The main protease (Mpro) of the betacoronavirus SARS-CoV-2 is an attractive target for the development of treatments for COVID-19. Starting from crystal structures of the Mpro in complexes with the Hepatitis C virus NS3/4A protease inhibitors boceprevir and telaprevir, we optimized the potency of the alpha-ketoamide boceprevir against the Mpro by replacing its P1 cyclobutyl moiety by a γ-lactam as a glutamine surrogate. In line with our original goal of identifying broad-spectrum inhibitors that target the main protease of coronaviruses and the 3C protease of enteroviruses, we also assessed the inhibitory potency of MG-78 against the Mpro of the alphacoronavirus HCoV NL63 and the 3Cpros of enterovirus A71 (EV-A71) and Coxsackievirus B3 (CVB3). Finally, coronavirus Mpros feature a catalytic dyad comprising a Cys…His pair, whereas enterovirus 3Cpros have a catalytic triad consisting of Cys…His…Glu(Asp).

Using 10 µM Dabcyl-KEALFQ↓GPPQFE(-Edans)-NH2 (↓ indicates the cleavage site) as a FRET substrate, we found IC50 values for MG-78 of 6.7 ± 2.2 μM against the EV-A71 3Cpro and 1.45 ± 0.40 μM against CVB3 3Cpro. Crystals of the EV-A71 3Cpro complex with MG-78 were grown in cubic space group P432 and yielded useful diffraction data extending to a Bragg spacing of 2.07 Å, whereas the CVB3 3Cpro complex gave crystals in space group C2 that diffracted to 1.65 Å. Compound MG-78 binds along the substrate-binding cleft in both proteases. Similar to the situation in the coronavirus Mpro, the nucleophilic attack of the catalytic residue (here Cys147) onto the α-keto group of the α-ketoamide warhead leads to the formation of a thiohemiketal, with a covalent bond between the sulfur of the catalytic Cys and the α-carbon. The amide oxygen of the warhead accepts hydrogen bonds from the Gly145, Gln146, and Cys147 amides of the oxyanion hole. The carbonyl of the γ-lactam accepts hydrogen bonds from His161 Nε2 and the side-chain hydroxyl of Thr142. In the CVB3 3Cpro structure, the contacts to Leu127 and Gly128 are more relaxed. Instead, there is a rather short distance to the Arg39 guanidinium group. The two nitrogens of the P4/P3 urea unit donate hydrogen bonds to the oxygen of Gly164 in the EV-A71 structure, whereas in the CVB3 protease, only one of these is strong enough to be called a hydrogen bond. Whereas the crystal structure of MG-78 in complex with the SARS-CoV-2 Mpro revealed an ideal fit, those of the complexes with CVB3 3Cpro and EV-A71 3Cpro demonstrated some steric incompatibilities that likely reduce the inhibitory potency. Such incompatibilities are more serious in the case of the EV-A71 3Cpro compared to the CVB3 3Cpro complex, in remarkable correlation with the inhibitory activities of MG-78 against the two proteases.

> GPAFEFAVAMMKRNSSTVKTEYGEFTMLGIYDRWAVLPRHAKPGPTILMNDQEVGVLDAKELVDKDGTNLELTLLKLNRNEKFRDIRGFLAKEEVEVNEAVLAINTSKFPNMYIPVGQVTEYGFLNLGGTPTKRMLMYNFPTRAGQCGGVLMSTGKVLGIHVGGNGHQGFSAALLKHYFN> KI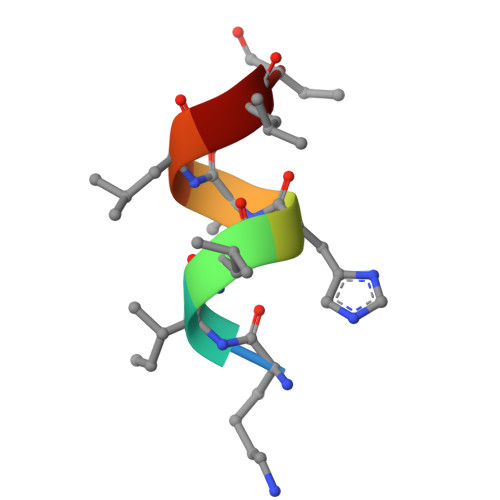LHRLLQ> MSLRRGIYHIENAGVPSAIDLKDGSSSDGTPIVGWQFTPDTINWHQLWLAEPIPNVADTFTL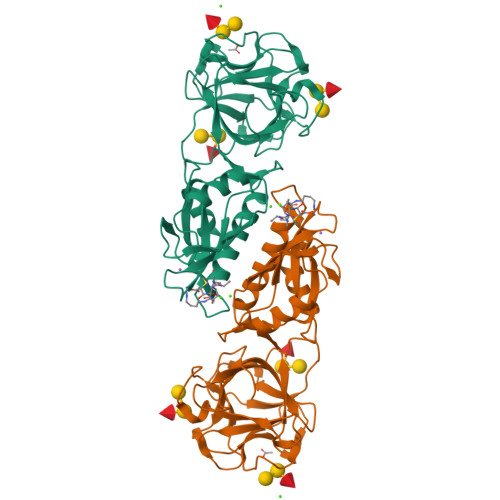ANLFSGTYMDLYNGSSEAGTAVNGWQGTAFTTNPHQLWTIKKSSDGTSYKIQNYGSKTFVDLVNGDSSDGAKIAGWTGTWDEGNPHQKWYFNRMSVSSAEAQAAIARNPHIHGTYRGYILDGEYLVLPNATFTQIWKDSGLPGSKWREQIYDCDDFAIAMKAAVGKWGADSWKANGFAIFCGVMLGVNKAGDAAHAYNFTLTKDHADIVFFEPQNGGYLNDIGYDSYMAFY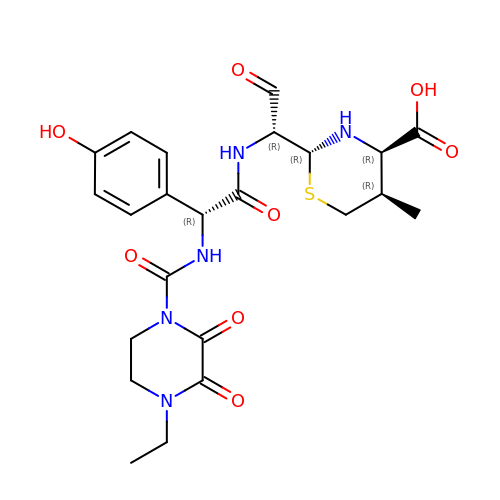(2R,4R,5R)-2-[(1R)-1-{[(2R)-2-{[(4-ethyl-2,3-dioxopiperazin-1-yl)carbonyl]amino}-2-(4-hydroxyphenyl)acetyl]amino}-2-oxoethyl]-5-methyl-1,3-thiazinane-4-carboxylic acid | C23 H29 N5 O8 S | XXVXTCZUKVAJAU-BMBOTXNISA-N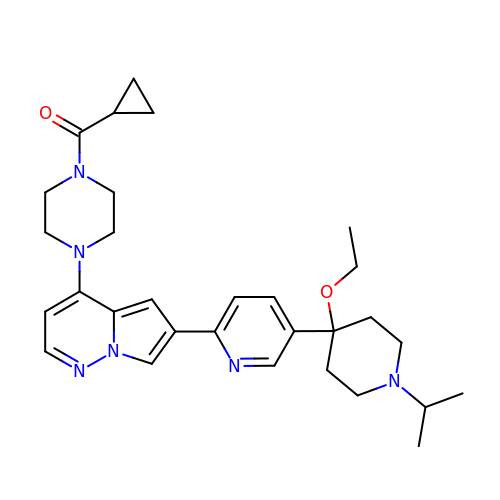cyclopropyl-[4-[6-[5-(4-ethoxy-1-propan-2-yl-piperidin-4-yl)pyridin-2-yl]pyrrolo[1,2-b]pyridazin-4-yl]piperazin-1-yl]methanone | C30 H40 N6 O2 | JQUZALVIPZBANO-UHFFFAOYSA-N methyl 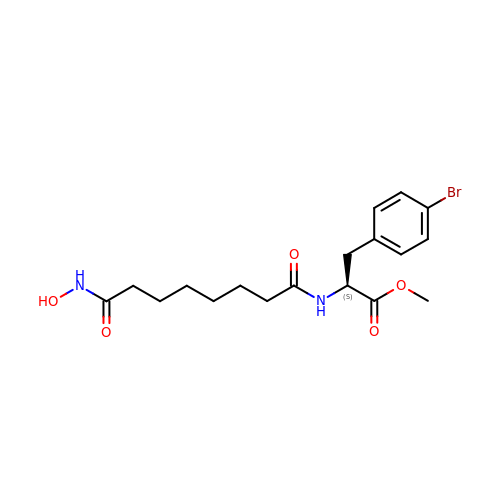4-bromo-N-[8-(hydroxyamino)-8-oxooctanoyl]-L-phenylalaninate | C18 H25 Br N2 O5 | UPYGSQPRAHMDPD-HNNXBMFYSA-N>MELDGDQMISHRELWAKIANSINDINEQYLKVYEHAVSSYTQMYQDFSAVLSSLAGWISPGGNDGNSVKLQVNSLKKALEELKEKYKDKPLYPANNTVSQEQANKWLTELGGTIGKVSQKNGGYVVSINMTPIDNMLKSLD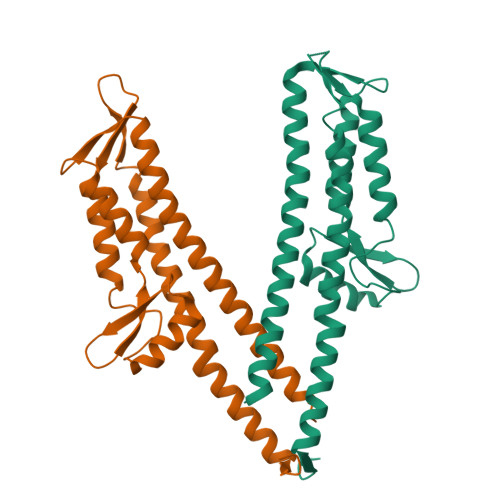NLGGNGEVVLDNAKYQAWNAGFSAEDETMKNNLQTLVQKYSNANSIFDNLVKVLSSTISS[2x]Centromeres are microtubule attachment sites on chromosomes defined by the enrichment of histone variant CENP‐A‐containing nucleosomes. To preserve centromere identity, CENP‐A must be escorted to centromeres by a CENP‐A‐specific chaperone for deposition. Instead, fly‐specific CAL1 appears to combine the roles of both HJURP and the Mis18 complex: pre‐nucleosomal CENP‐A recognition and its targeting to the centromere for deposition, respectively (Phansalkar et al, 2012). In this study, we present the structural basis for the recognition of CENP‐A/H4 and CENP‐C by CAL1.

The structure of CENP‐C1264–1411 bound to CAL1841–979 was determined by molecular replacement using the CENP‐C1264–1411 structure reported here as a search model. CENP‐C binds CAL1 using a cradle‐shaped surface formed by loops L1, L2 and L3 and β‐strands β1 and β2. The calculated electrostatic surface properties show that CAL1 binding involves a surface suitable for both electrostatic and hydrophobic interactions. CAL1 residues 890–893, which form a β‐strand, interact with β1 of CENP‐C cupin domain running parallel to it and as a consequence extend the β sheet involved in cupin dimerisation. The CAL1 α helix consisting of residues 894–913 makes several hydrophobic (involving L896, I900, W904 and Y908) and electrostatic (R903 and K906) interactions with a complementary hydrophobic (involving residues Y1315, V1317, Y1322 and F1323) and acidic (S1295, E1311 and N1326) region of the cradle‐shaped CENP‐C surface. To evaluate the requirement of these interactions to stabilise CAL1–CENP‐C binding, we mutated conserved CENP‐C F1324 to Arg and CAL1 I900 to Arg and K907 and Y908 to Ala and tested the ability of these mutants to bind wild‐type CAL1 and CENP‐C, respectively, in separate SEC experiments. Both His‐CENP‐C1264–1411 F1324R and His‐SUMO‐CAL1841–979 I900R/K907A/Y908A failed to interact with His‐SUMO‐CAL1841–979 and His‐CENP‐C1264–1411, respectively, and hence eluted at their original elution volumes as compared with the elution volume of the CENP‐C–CAL1 complex. In the crystal structure presented here, the CAL1 binding site on CENP‐C is in close proximity to the cupin dimerisation interface: the loop L1 and β‐strands β1, β2 and β3 are all directly involved in stabilising the cupin dimer. Although CAL1 binding by CENP‐C involves just a cupin monomer, only one of the two cupin monomers was observed to interact with CAL1, while the equivalent CAL1 binding site of the dimeric counterpart was empty in the crystal structure. We speculate that the other binding site might be sterically hindered by the remaining residues of CAL1 not seen in the crystal structure, thus not allowing a second monomer of CAL1 to bind. Thus, the AUC together with the crystal structure shows that CENP‐C cupin dimer binds just one copy of CAL1 at any given time.

>[4x]MSKPQNNDTLELDDILSQPVKDKERFAAFMMRKLAENKPAQNDNLFGNFKLDFDLDFEVPLIKKSQAKPKSKLPEVQPLGELVSKNSAATEKVNEPPVDQAPNENVPPRRSPTLSPNNRRSMRRSGNVPGSDKLRRHAIRRRSRSCGRQLLPEFEETVNLTRSISSPVNFLPEISSTPCTEKQKEEVAKNTTRVETDKPAEKPMELSQEPEPENPLQTKVTSPARNPILAAEIEQICKERQSSFHKNVLQLDYSGRAPYSRPPTPSSPSVAGLRRTYTMEKGPAPGQLLLSPSHRYDTPSKMPVVKAKRFNQELMVPDTPERQSHDPAWQSEPQPEFVVPETQPQDLGELVQTLSRSAISPIVVINTSNSNRSVRRDAVAMKSVPTSPVTALSSPPIAPSPRRSAAASPQKSIAQLPRVEENMDAIMTDDESDEHPSTVPLNLAPSGGNTTRQRRLRSSNRARATIESQESSMRLLNLHKSVNAKKSKPRKTAIPLNKAPSAPINGEQFARELTRMSNYEILDLRKRNSLNEIYPLNGHRNHRSEKLILEEEIQRELLRRNLMDEAEGLPKQQSSDDSNEDYIPVPPKTQSLRTKSNDRSQGRGRPRSTRRDLPMTTELVNYLGLSQTLETRRKSSKDGKRCLYTKGSSDHEDNDSLSPVKLPRLSKSIQIVPPPPVSLRYSQSLQNLPCSGKFDFDNVVMAAPPDFHDSVNSDAIEIAPPPPEYVVNTRGRSTSGRKSNKNDLVLPPPGYEGGQEEEHDERPSQPRCTAKELQQSTQNGRRAMENELVPPPIEYVEEENRNNEQSRRSTKNGNLVDRNTHNAVEYCEPPEPPEYDDSDHGQASILRRSGKKLQHSKQSVQKSNKEQIIAPSYENNEDYDSDEEPIYNEEYGKEESQNKNVTRRKSDKDEMASHTLECIEGPDPNWNSSCNKQNRNHQNASKSKENDKLANRSSKSQKLSNPRQNAVGTEKSVALSNRGEECTEKSSDVMESLRVNTPTPPIDQNSDDVPSRNPSPSRTLLSDDVPSTSRAALEFLQRSQNMSKSRPPDESSADVVFKKPLAPAPRAKSKKGKSEVDKLKLAKMPVEAEELNTTGIRRSKRGQVPLQMSWCHTMDPSKFNFMSGFIEPRSKNSKTKKGNLSKAKKASATKPKPTVEKNLPDNRGPLCSSTPRISEKLPGAIPHSESLGLSTLTWEETEVQAEAEKVPKKRGRPKKAVGGVQTDTEAEPEPEPEPMISSVAPLTSDQEEPDVPDEQAPYTEAALGPVVFSTPLRDEQEEASTKLMQWLRGVGDAPPSASMSDENASVSSANELIFYQVDGIDYAFYNTKEKAMLGYMRFKPYQKRSMKQAKVHPLKLLVQFGEFNVETLAVGEEKEVHSVLRVGDMIEIDRGTRYSIQNAIDKVSVLMCIRS;> MANAVVDEETLEAMVYERSKAWSSKMADFASLEDGMEIDVAEFDNLFHGEDEDPDLDDVAKEAVEDNVPDEAKLEMGHINATSVTELTLILCANEDNEAKAEIEEILNQTVPVVEEHKRKWREAGLDRILDTFDEKQIEHHVGRWMRRHNSVYLEASPPKYLPPHHNSISDESDESMHSIDTARYIQQSRRRNAHMTNKNMTTIKMYRKHSHKRDELRAKYAYGDEQEHRHHMQAVLLRRRERERQLAYLASTPMQCVYSSGHHMRRKNLRKRRINSWMFDSASSSEEDTSFGGCDCHSCRRHYALSRSVYQSCPYGRGQREYHHRQMASRTMHTMRRQHTFDMEMDLRPRLPENECSCCNSDRLCSNVIHIANSSTEEWVVENRSNHLTQETQEKTRKQKHQPMDARKVSHQPVCSKGHEQKPLSSKATSVSKLVLSKEKYMQMFDSESSDEDNALAKKGLLCCSDKKKGMTFPTPNAAGKITHPTSSAKKAIRKEARPNGLAQIQEEGPTATNSPIESTYLPVAHMKSVSIDGSSGTSATFESPAKKAPKRGIRETSPLNGNELQQLISTIPIADEKASSLMEKVDNCIGRESFDDRNKDFMHMENSSTKTAVEKSTKQKRVSGKKSEIPKSIITNNEILEKNSTETLSEKQVAAKAKKQSVRKTGATGKPSTSRLKKSEKTKTTSSVTSTSKLEQVREEESDVSSEVLAKPKPQCSTTASILKQGGDGASNSEDDLQIALAMSKATYKEEQQKRKKTKREPSNKQPQSPAEKSMTVFNNQSVACNSTALANDTACYRVLPKRRGVKRAAAVSTTEEKTATNSSSSPTSSLEEMGSPTGGDPDCTVVTSTTGCEPPASERQEIPATIKITKRGILLHSPSAPEGASFTLTEQGLGKIIGERWARKYLKYHIGSRSFDSRHSVYYQPTPQLAAALSAPQDAQNIGNISGSSASDDDIFEQINRYGTVYSILENNSGDK>MALVDLVRAGGYSVEYPQFSSMAKLKAFPHSEDGQLVRLLSWHEGVGLGGGLFKVSTSSTATGNDGTVVVASNGVRLLRVVNGPIWADMFGALPNSDIDSMPAVAAAYAYAASVNTDLYIGVATYKFKGSTPINVDPSRAGIIGYQGKVRIDCSEFTGSIVFSINSSYSYTPAAYYNNLSPALQGLYVFGAKTSGVDGLLVGRETVGSDKSYNGQTEVRECTFDKFDRNIRMGHNSWRFVFYKVNSLNALSPNGILYVPAGLDDSGEILSFYHCQFFDGAGSNIRLSCSSYTMVFNTCSFLNITFFVDSASSATVTCNGCNFENPGSASTRRYVDISAGHTNVFNIIGGSIVTNSNPGQTQALLYVSTDNLLNLVGVTAPYGGHYQQEQELGYHAFIGGAGTVTTSGVMLQLRNGAGTCPLHSSLSTFSNWNFGYGNLNAWTVDKG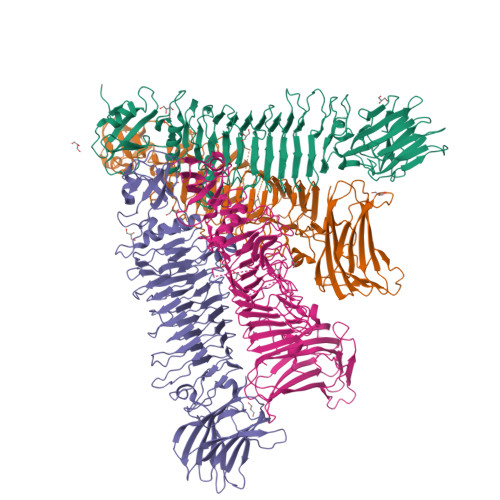TGTSSVVEYLANAGPKGTEGAMRVAPVSVGTNVSQVQAVTNPGMFSMSCMVNIATTPGNAGQVSIGFLDAAGNSLPGGVSANLGTTTGWQVIGKNTLRGKVPIGAKQVRVNIQTVAGADVKYAYLLCNVVKPLEHHHHHH[4x]7-(2-(2-(2,4-dioxo-3,4-dihydropyrimidin-1(2H)-yl)ethoxy)phenoxy)-2-naphthonitrile 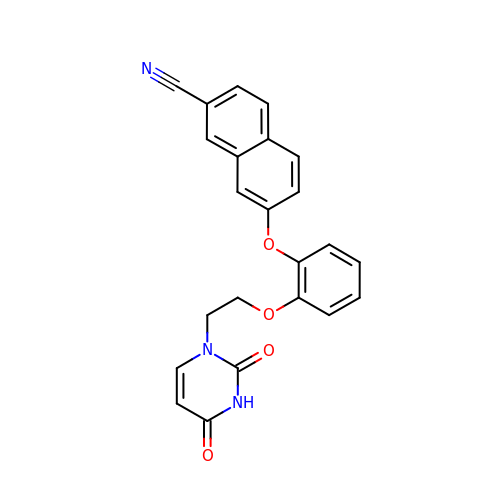| C23 H17 N3 O4 | KULHKTUYJZTZIY-UHFFFAOYSA-N> GPLGSETITVPTPIKQIFSDDAFAETIKDNLKKKSVTDAVTQNELNSIDQIIANNSDIKSVQGIQYLPNVTKLFLNGNKLTDIKPLANLKNLGWLFLDENKVKDLSSLKDLKKLKSLSLEHNGISDINGLVHLPQLESLYLGNNKITDITVLSRLTKLDTLSLEDNQISDIVPLAGLTKLQNLYLSKNHISDLRALAGLKNLDVLELFSQECLNKPINHQSNLVVPNTVKNTDGSLVTPEIISDDGDYEKPNVKWHLPEFTNEVSFIFYQPVTIGKAKARFHGRVTQPLKEVYTVSYDVDGEVIKTKVEAGTRITAPKPPTKQGYVFKGWYTEKNGGHEWNFNTDYMSGNDFTLYAVFKAET

InlB, an invasion protein from the facultative intracellular pathogen Listeria monocytogenes, is a multi-domain protein that binds and activates the human receptor tyrosine kinase MET. The N-terminal internalin domain (amino acids 36–321; InlB321) is characterized by a central leucine-rich repeat (LRR) region that binds to the first Ig-like IPT domain of MET with high affinity. The LRR region is flanked N-terminally by a helical cap and C-terminally by an Ig-like inter-repeat (IR) region. The B repeat folds into a compact domain resembling a β-grasp fold.

InlB392_T332E, an InlB392 variant with a single Thr-to-Glu substitution in the B repeat, readily yielded single crystals of varying morphologies in several conditions from the commercial MORPHEUS screen and a homemade PEG smear screen. The best crystal from condition D3 of the PEG smear (low- and broad-molecular-weight) screen (crystal form II) was a rod with a cross section of about 35 × 35 µm and a length of about 180 µm. This crystal diffracted to 1.8 Å resolution. The packing of InlB392_T332E crystal form II is different. The contact area is between 397 and 647 Å2, with a mean of 549 Å2, according to the PISA server. This crystal contact is not present in crystal form II of InlB392_T332E. The largest difference between these distances is found for InlB392_T332E crystal form II. The crystal structures presented in this work provide additional and conclusive proof that the T332E mutation does not change the structure of the B repeat. Therefore, the negative effect of this substitution in cellular assays is most likely due to the destruction of a binding site, preventing the interaction with a functionally important binding partner. Secondly, the contact between the B repeat and the IR region is formed regardless of the T332E mutation.>[2x]MSGEEAVRRRFEELLREALAFRERTGGRRETLEHAVRLARELAEFAASH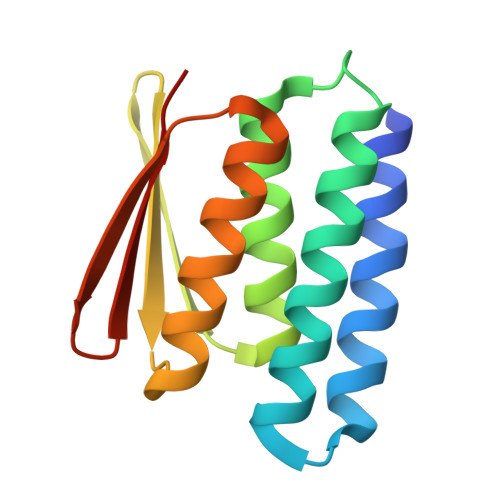PEFNRQEAVLLAIELMVRAMGVTMETHRSGNEVKVVIKGLNIDEQRALYRAVRETSKIMGVETEIEVEGDTVTIVVREGSG>MNGTAEERNKFDKLDPYFQQGWFHFQKSLYYISSVKNTWHLSREYCLQEGADLAIINSRAEQAFLENFKMTLWIGLMEQRSERTWRWVDGTPLTESYWSLGEPNNYEGRQEQCVEQIDREDKKGWNDLVCEFSNFYMCEKRIFP[2x]

Among such receptors is macrophage-inducible C-type lectin (Mincle, gene symbol CLEC4E), a member of the C-type lectin receptor (CLR) family, which functions as an immune sensor for both pathogens and damaged self. Mincle recognizes its ligands via a calcium-dependent sugar-binding site, containing a conserved EPN (Glu-Pro-Asn) motif, and a hydrophobic groove on the carbohydrate recognition domain (CRD), which are in combination the major characteristics of Mincle. In Takifugu rubripes, one of the first vertebrates whose whole genome was completely sequenced, a protein sequence bearing the EPN motif and a hydrophobic groove was found (XP_029706534.1). Altogether, trMincle shares similar characteristics with mammalian Mincle in its amino acid sequence and its FcRγ-dependent cell surface expression.

As the structural analysis suggested that trMincle possesses a sugar-binding pocket, we set out to investigate the sugar recognition mechanism using monosaccharide glucose as a candidate for the model ligand. Indeed, the crystal structure of the trMincle CRD-glucose complex was determined at 1.8 Å resolution. As suggested by the glycerol complex, one glucose molecule interacted with the calcium ion as well as the surrounding side chains. Thus, the sugar-binding mode of trMincle was similar to the other CLRs bearing EPN motifs. Indeed, computational superposition of the boMincle-trehalose complex onto the trMincle-glucose complex demonstrated that trehalose causes a heavy steric clash with trMincle, suggesting that trehalose disaccharide cannot bind to trMincle due to the narrow pocket. It evokes the possibility that trMincle cannot recognize disaccharide-bearing glycolipids, which are typical of exogenous origin, such as mycobacterial glycolipids (e.g., TDM or trehalose monomycolate (TMM)), but instead may only bind monosaccharide-bearing glycolipids, which are often derived from self, like β-GlcCer. While mammalian Mincle recognizes both exogenous diglycosylated lipids and endogenous monoglycosylated lipids, our results imply that trMincle may function as a receptor that selectively binds ligands such as monosaccharide-bearing glycolipids. The narrow sugar-binding pocket of trMincle suggests specialized recognition for monosaccharides. This makes it difficult to recognize well-known mammalian Mincle ligands such as mycobacterial glycolipid TDM. Although trMincle may not have the ability to recognize typical mycobacterial glycolipids like mammals, it may detect fatal infection through the alteration of endogenous metabolites, such as hexosylceramides.ethyl 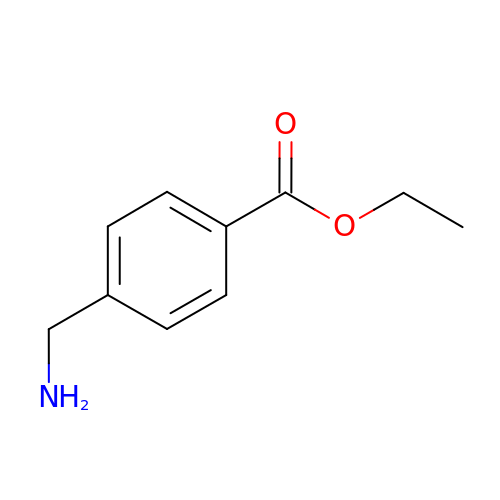4-(aminomethyl)benzoate | C10 H13 N O2 | WCTQEHGXBKFLKG-UHFFFAOYSA-N>MSSSHHHHHHMPTKKQKSKSKLKPFFALVRRTNPSYGKLAFALALSVVTTLVSLLIPLLTKQLVDGFSMSNLSGTQIGLIALVFFVQAGLSAYATYALNYNGQKIISGLRELLWKKLIKLPVSYFDTNASGETVSRVTNDTMVVKELITTHISGFITGIISVIGSLTILFIMNWKLTLLVLVVVPLAALILVPIGRKMFSISRETQDETARFTGLLNQILPEIRLVKASNAEDVEYGRGKMGISSLFKLGVREAKVQSLVGPLISLVLMAALVAVIGYGGMQVSSGELTAGALVAFILYLFQIIMPMGQITTFFTQLQKSIGATERMIEILAEEEEDTVTGKQIENAHLPIQLDRVSFGYKPDQLILKEVSAVIEAGKVTAIVGPSGGGKTTLFKLLERFYSPTAGTIRLGDEPVDTYSLESWREHIGYVSQESPLMSGTIRENICYGLERDVTDAEIEKAAEMAYALNFIKELPNQFDTEVGERGIMLSGGQRQRIAIARALLRNPSILMLDAATSSLDSQSEKSVQQALEVLMEGRTTIVIAHRLSTVVDADQLLFVEKGEITGRGTHHELMASHGLYRDFAEQQLKMNADLENKAG[2x]

The Bacillus subtilis efflux pump BmrA, belongs to the type-IV family of MDR ABC transporters, conferring resistance to cervimycin-C secreted by the biotope competitor Streptomyces tendæ13. Type IV ABC transporters involved in MultiDrug Resistance (MDR) phenotype perform their function by undergoing a series of conformational changes pertaining to the alternating access mechanism. They are formed of two transmembrane domains (TMD) forming a cavity at their center where substrates bind, and of two nucleotide-binding domains (NBD) binding and hydrolyzing ATP-Mg2+ to fuel the system. Binding of ATP-Mg2+ to the NBDs bring them together, translating this conformational change to the TMDs which then open towards the outside (Outward-Facing, OF) where substrates are released. Importantly, the E504A catalytic mutant that still binds ATP but cannot hydrolyze it20 was used in this study; this thus allowed to probe a unidirectional transition from IF to OF states, BmrA being blocked when reaching the OF conformation when complexed with ATP-Mg2+ 9,12,14.

CryoEM grids were frozen at key ligand concentrations and imaged; without ATP-Mg2+ in absence or presence of R6G (named E504Aapo and E504AR6G), at a 1:1 molar ratio ATP-Mg2+:BmrA dimer (E504Aapo-25µMATP and E504AR6G-25µMATP), at the K0.5 or close to the Kd-app for ATP-Mg2+ (E504Aapo-100µMATP and E504AR6G-70µMATP), and at saturating concentrations of ATP-Mg2+ (E504Aapo-5mMATP and E504AR6G-5mMATP). Clear electron densities could be observed for R6G in all the IF and OF reconstructions where it was added. In the IF conformations, R6G could also be modeled within the TMD in-between the same TM helices. Here again, electron density denotes multiple positions adopted by the molecule (also observed in MD simulations below), in line with the ability of BmrA to recognize structurally-unrelated ligands. R6G binding in E504AR6G and E504AR6G-25µMATP results in a further rearrangement of TM helices within the dimer, with a wider opening of TM4-5-6’. Surprisingly, the rearrangement does not occur within a half-transporter, as it overlays well with BmrA in absence of R6G, but in the relative orientation of the two halves (right part of the structure on which the overlay is performed). The effect of R6G binding further translates all the way to the NBD, resulting in a reorientation of the 2 NBD that face each other more directly, hinting at an influence on ATP binding observed in Fig. 1. The first NBD rotation centered on V363 is conserved in E504AR6G, while the rotation centered on E453 is reduced by more than half. Notably, the oscillation that bring the NBDs closer together is greatly affected as the E504AR6G structure is stiffened and movements are very reduced (less than 1 Å). However, the conformational space explored by E504AR6G is much more focused compared to E504Aapo in which the NBDs explore a larger space, hinting at the allosteric influence of R6G on the NBDs.In the present study, we report a novel type of CAs that has been characterized in the eukaryotic microalga Bigelowiella natans and the cyanobacterium Anabaena sp. PCC7120. Taken together, these results suggested that the COG4337 proteins are metal-free enzymes that catalyze the hydration of CO2 to HCO3-, but not the reverse reaction. Each domain formed a cone-shaped barrel structure comprising three α-helices and a four-stranded antiparallel β-sheet, which were almost identical across the COG4337 domains of Bn86287 and all2909. We thus concluded that COG4337 proteins should be treated as a new variant of ι-class CAs.

To further analyze the metal-free catalytic mechanism of COG4337 proteins, crystal structures of Bn86287 and all2909 were determined. Crystallographic analysis was performed using crystals soaked in solutions with bicarbonate and the anion inhibitor iodide; the addition of 1 mM KI led to the deactivation of the COG4337 proteins. Iodide ions have been reported as an inhibitor in several classes of CAs. The substrate (bicarbonate) and inhibitor (iodide ion) were found in a bent finger-like cavity of the cone-shaped barrel. As expected from the biochemical assays described above, electron densities corresponding to metals were not detected in the cavity. Considering that hydroxyl groups of Thr106/159/322/486 (residue numbers in all2909/1st/2nd/3rd domain of Bn86287) and Tyr124/176/339/503 were found at a distance of 2.5 to 3.5 Å from an oxygen of HCO3- and at a distance of 3.2 to 3.7 Å from an iodide ion, these hydroxyl groups would most likely mediate the deprotonation of active site water. Similarly, an iodide inhibitor was reported to be positioned 3.6 Å from the hydroxyl group of Thr199 in hCAII. The results of size exclusion chromatography with multi-angle static light scattering (SEC-MALS) system showed that Bn86287 exists as dimers but all2909 exists as tetramers in solution. Analysis with the PISA (Protein Interfaces, Surfaces and Assemblies) software estimated that a tetramer of all2909 was assembled by a head-to-head interaction of two dimeric units. Notably, Lys180 in all2909 was found at the analogous position of Tyr224/388/552 in Bn86287.

>GSHDSGDKITATSSLKTPIVNRAITESEVLAAQKAWGEALVAISTTYDAKGKASAKALAEKVIDDAYGYQFGPVLFKPTLAISPRTFRTTRAGALAYFVGDDKAFPEDKGFALSSWRKVEIKNAAIFITGNTATTMGNVIITDKQGKATTVDKTWQFLKDDHGKLRIITHHSSLPYEQ[2x]Interestingly, the type I-D system utilizes subunits that are homologs of type I complexes, type III complexes, or both. The type I-D operon contains the type I signature gene cas3 split into its two domains; the helicase domain (Cas3′) encoded from a stand-alone gene, and the HD nuclease domain (Cas3″), which is fused to the large subunit as part of the core effector complex. The Cas10d subunit is bigger than other type I large subunits (Cas8) and similar to type III large subunits, yet retains the type I functionality of discerning PAMs in target DNA sequences. As is typical for Cascade complexes, a repeating, helical backbone of Cas7d subunits assembles around the crRNA, while the C-terminus of Cas10d and two Cas11d subunits constitute a minor filament along the belly of the complex.

To investigate ssRNA binding and single-stranded vs double-stranded target discrimination by type I-D Cascade, we bound type I-D to a ssRNA target containing a protospacer that matched the crRNA spacer and performed cryo-electron microscopy. Our efforts resulted in a structure of the ssRNA-bound complex at 3.1 Å resolution. Overall, the structure is strikingly similar to the double-stranded target-bound complex. However, in the single-stranded target-bound complex, we lose recognizable density for the PAM recognition domain, likely due to the flexibility of this subunit in the presence of a single-stranded nucleic acid. We propose that the lack of a distinct dsDNA PAM in the ssRNA allows the PAM recognition domain to remain unlocked and inactive (PRD disengaged). Our structural studies revealed a flexible PRD in the ssRNA-bound complex, which suggests that the type I-D Cascade does not require PRD engagement with a specific protospacer flanking sequence for ssRNA binding. Indeed, binding of a ssRNA substrate containing either a 5′-AAC-3′ PFS (corresponding to the complement of the GTT PAM) or a scrambled PFS (5′-ACG-3′) showed nearly identical binding with an apparent affinity of 11.0 ± 0.9 nM. We observed no binding to a non-specific control ssRNA that lacked complementarity to the crRNA. Single-stranded target-bound Cascade has a flexible PRD (PRD disengaged). Based on this structural analysis, there is no indication that AcrID1 binding to type I-D Cascade would affect single-stranded nucleic acid binding, consistent with SIRV3 being a dsDNA virus.

>[7x]MLDSLKSQFQPSFPRLASGHYVHFLMLRHSQSFPVFQTDGVLNTTRTQAGLLEKTDQLSRLVMFKRKQTTPERLAGRELLRNLGLTSADKSAKNLCEYNGEGSCKQCPDCILYGFAIGDSGSERSKVYSDSAFSLGAYEQSHRSFTFNAPFEGGTMSEAGVMRSAINELDHILPEVTFPTVESLRDATYEGFIYVLGNLLRTKRYGAQESRTGTMKNHLVGIVFADGEIFSNLHLTQALYDQMGGELNKPISELCETAATVAQDLLNKEPVRKSELIFGAHLDTLLQEVNDIYQNDAELTKLLGSLYQQTQDYATEFGALSGGKKKAKS;> MTKIYRCKLTLHDNVFFASREMGILYETEKYFHNWALSYAFFKGTIIPHPYGLVGQNAQTPAYLDRDREQNLLHLNDSGIYVFPAQPIHWSYQINTFKAAQSAYYGRSVQFGGKGATKNYPINYGRAKELAVGSEFLTYIVSQKELDLPVWIRLGKWSSKIRVEVEAIAPDQIKTASGVYVCNHPLNPLDCPANQQILLYNRVVMPPSSLFSQSQLQGDYWQIDRNTFLPQGFHYGATTAIAQDSPQLSLLDTN;> MTTLLQTLLIRTLSEQKDYILLEYFQTILPALEEHFGNTSGLGGSFISHQKHFGTQGYDTEKAKKMAQGFAKKGDQTLAAHILNALLTTWNVMQELEFPLNDIERRLLCLGITLHDYDKHCHAQDMAAPEPDNIQEIINICLELGKRLNFDEFWADWRDYIAEISYLAQNTHGKQHTNLISSNWSNAGYPFTIKERKLDHPLRHLLTFGDVAVHLSSPHDLVSSTMGDRLRDLLNRLGIEKRFVYHHLRDTTGILSNAIHNVILRTVQKLDWKPLLFFAQGVIYFAPQDTEIPERNEIKQIVWQGISQELGKKMSAGDVGFKRDGKGLKVSPQTSELLAAADIVRILPQVISVKVNNAKSPATPKRLEKLELGDAEREKLYEVADLRCDRLAELLGLVQKEIFLLPEPFIEWVLKDLELTSVIMPEETQVQSGGVNYGWYRVAAHYVANHATWDLEEFQEFLQGFGDRLATWAEEEGYFAEHQSPTRQIFEDYLDRYLEIQGWESDHQAFIQELENYVNAKTKKSKQPICSLSSGEFPSEDQMDSVVLFKPQQYSNKNPLGGGQIKRGISKIWSLEMLLRQAFWSVPSGKFEDQQPIFIYLYPAYVYAPQVVEAIRELVYGIASVNLWDVRKHWVNNKMDLTSLKSLPWLNEEVEAGTNAQLKYTKEDLPFLATVYTTTREKTDTDAWVKPAFLALLLPYLLGVKAIATRSMVPLYRSDQDFRESIHLDGVAGFWSLLGIPTDLRVEDITPALNKLLAIYTLHLAARSSPPKARWQDLPKTVQEVMTDVLNVFALAEQGLRREKRDRPYESEVTEYWQFAELFSQGNIVMTEKLKLTKRLVEEYRRFYQVELSKKPSTHAILLPLSKALEQILSVPDDWDEEELILQGSGQLQAALDRQEVYTRPIIKDKSVAYETRQLQELEAIQIFMTTCVRDLFGEMCKGDRAILQEQRNRIKSGAEFAYRLLALEAQQNQN;>[2x]MTEKLKLTKRLVEEYRRFYQVELSKKPSTHAILLPLSKALEQILSVPDDWDEEELILQGSGQLQAALDRQEVYTRPIIKDKSVAYETRQLQELEAIQIFMTTCVRDLFGEMCKGDRAILQEQRNRIKSGAEFAYRLLALEAQQNQN> SMQEEDTFRELRIFLRNVTHRLAIDKRFRVFTKPVDPDEVPDYVTVIKQPMDLSSVISKIDLHKYLTVKDYLRDIDLICSNALEYNPDRDPGDRLIRHRACALRDTAYAIIKEELDEDFEQLCEEIQESR

Bromodomain-containing proteins are a prominent class of epigenetic readers that recognize acetylated lysine residues, typically on histones. BRD4, a member of the bromodomain and extraterminal subfamily, which in fact contains two bromodomains, is perhaps the most widely studied family member and has been shown to be very amenable to binding druglike molecules. ATAD2 was proposed from computational druggability analysis to be less tractable than BRD4, attributed in part to it lacking the hydrophobic region present in the BRD4 ligand binding site, termed the “WPF shelf”, interactions with which are postulated to contribute significantly to ligand binding affinity. We demonstrate the utility of FragLites in mapping the binding sites of bromodomain proteins BRD4 and ATAD2 and demonstrate that FragLite mapping is comparable to a full fragment screen in identifying ligand binding sites and key interactions.

The remaining hits for ATAD2 (13/16) and BRD4 (9/26) were bound in allosteric pockets of their respective proteins. However, a halogen bond constitutes the primary interaction (other than lipophilic interactions) in the absence of a hydrogen bond only for FL10 and 23 in ATAD2, and FL2, 4, 21, and 24 for BRD4. In both ATAD2 and BRD4, while the majority (22/42) of binding events involved ligands that contacted only one molecule, a significant fraction (FL2, 4, 5, 7, 10, 11, 12, 15, 19, 21, 22, and 24 in BRD4 and FL1, 2, 6, 7, 10, 28, and 29 in ATAD2) were involved in contacts with more than one protein molecule in the lattice. As such, the hits for these FragLites may not occur in solution.>MLTQHVSEARTRGAIHTARLIHTSDLDQETRDGARRMVIEAFRDPSGDSDFTDDFTDDDWDHALGGMHALISHHGALIAHGAVVQRRLMYRGPDGRGHALRCGYVEAVAVREDRRGDGLGTAVLDALEQVIRGAYQIGALSASDIARPMYIARGWLSWEGPTSVLTPTEGIVRTPEDDRSLFVLPVDLPDGLELDTAREITCDWRSGDPW[4x]

Three different classes of enzymes are well established: ATP-dependent phosphotransferases (O-phosphorylation, APH), ATP-dependent nucleotidyltransferases (O-nucleotidylation, ANT), and acetyl coenzyme A (CoA)-dependent N-acetyl-transferases (N-acetylation, AAC). Here, we present the crystal structures of an AAC(2′) from M. smegmatis [AAC(2′)-Id] in its apo-form and AAC(2′)-Id complexed with CoA and different aminoglycosides (gentamicin, sisomicin, neomycin, and paromomycin). Collectively, the kinetic results indicate that AAC(2′)-Id has a very broad substrate-binding specificity, similar to AAC(2′)-Ic9. AAC(2′)-Id was not active on streptomycin because the antibiotic does not contain 2′ amino groups in its chemical structure, indicating that AAC(2′)-Id exhibits strict regioselectivity.

The asymmetric unit of the apo-AAC(2′)-Id structure comprises a dimer of dimers. The final model of apo-AAC(2′)-Id contains 742 amino acid residues (dimer of dimer, subunit A: 191 residues, subunit B: 180 residues, subunit C: 184 residues, subunit D: 187 residues), whereby the N-terminal loop region (residues 1–14) and the 45–51 loop region are commonly missing due to weak electron density in all subunit structures. The monomer structure of apo-AAC(2′)-Id has one long β-sheet surrounded by four α-helices. The dimerization of apo-AAC(2′)-Id is achieved by interactions among β1, α2–β2 loop, β3, β4, α3, β7–β8 loop, and β10. Moreover, the dimerization of apo-AAC(2′)-Id was confirmed in solution via analytical ultracentrifugation. Structural comparison between the apo- and the substrate-CoA-bound AAC(2′)-Id structures revealed significant conformational differences in the α1–α2 loop, α4-helix, and β8–β9 loop region between the structures. The α1–α2 loop is the most flexible region in the structure of AAC(2′)-Id and thus misses some residues. This loop may move and cover the substrate-binding site in the apo-structure, whereas it exhibits a more open conformation in the substrate-bound AAC(2′)-Id structures. In the apo-AAC(2′)-Id structure, Arg179 forms a salt bridge with Asp208 and Asp177, as well as hydrogen bonds with the carbonyl oxygen atom of Trp210. The salt bridge, however, is lost in all substrate-bound structures as Arg179 flips away from Asp208 and Asp177.>[2x]SNVRATYTVIFKNASGLP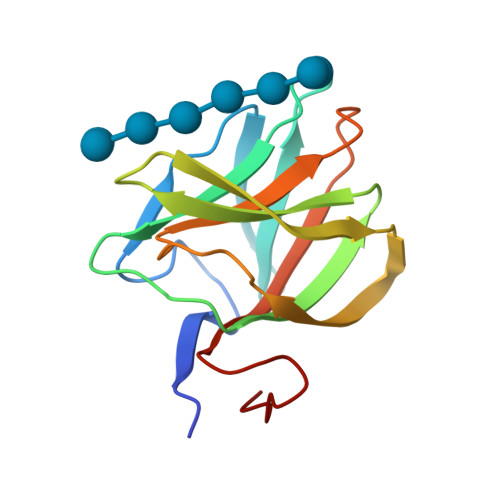NGYDNWGWGCTLSYYGGAMIINPQEGKYGAVSLKRNSGSFRGGSLRFDMKNEGKVKILVRNSEADEKFEVETISPSDEYVTYILDVDFDLPFDRIDFQDAPGNGDRIWIKNLVHSTGSADDFVDPI N-(2,2-dimethylpropyl)-N~2~-[4-(hydroxycarbamoyl)benzene-1-carbonyl]-L-asparaginyl-N-benzyl-L-alaninamide 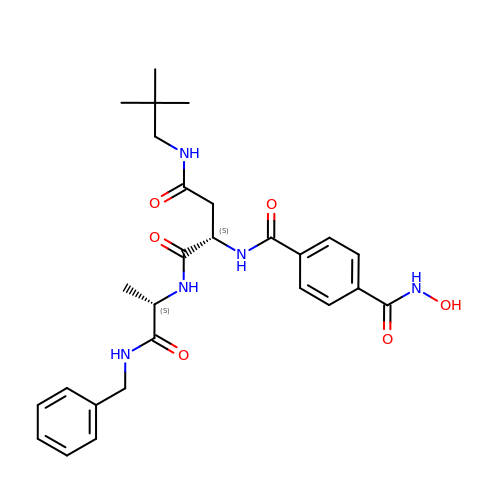| C27 H35 N5 O6 | CMINWSPSBRREEO-UWJYYQICSA-N> MPMISCDMAYGRTDEQKRALSAGLLRVISEATGEPRENIFF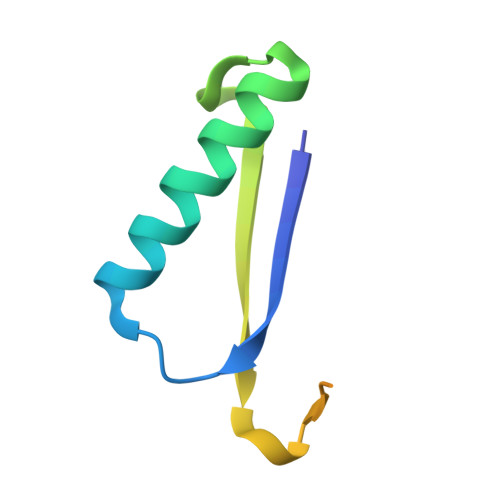VIREGSGINFVEHGEHLPDYVPGNANDKALIAKLK>MSTVAVTDATFEADVLKSSKPVLVDFWAEWCGPCKQIAPALEQLSEELADVVTIAKVNIEDSPTTPSRYGVRGIPTMMLFRDGQMTSMKVGAMPKQ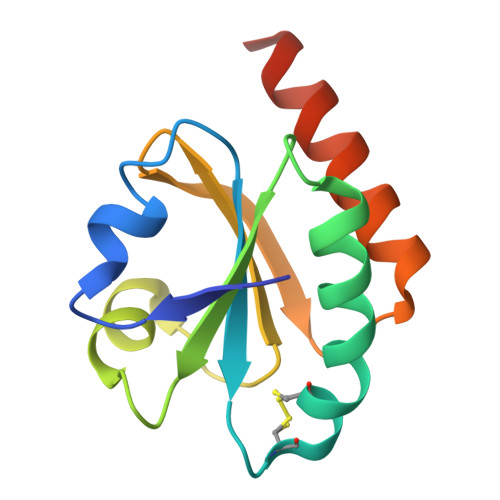KILEWLNEAGVQAALEHHHHHH[3x]> RLGIV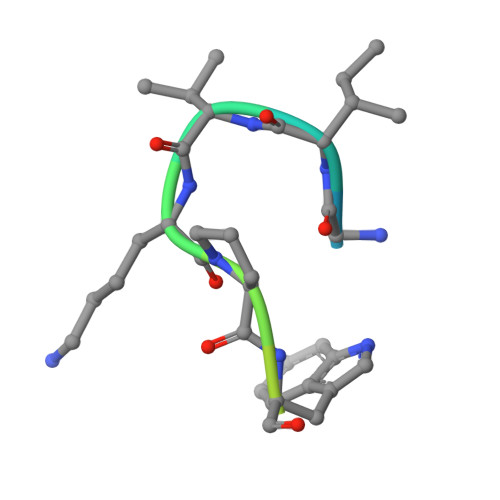KPWNSTWFANX>[27x]MSVHALRELFKHKGEKNYEVFSMEDFIGRLESEIGLNDSVVSQGRSLISSISHENFGTVQATDIQDAAAIYNKMQMLVNDYGFERVSSSDPQVRAREERVRENQITAATMAAIACADETKYIRALRGITKAKASNEDHVKVVQHQFNGPAGGIQVFENGVGLENYNEKSQRDFRVVTIGYNLAASRQDEFAERIYPTTVINPIEGGVVQVLPYIAVMKDVYHEVSGVKMDNEEVNMVEAYRDPSILDDESIALIPALDPAGSNADFFVDPALVPPYTIKNEQNLTITTAPLKANVRLDLMGNSNANLLIQRGMLEVSDTIDPAGRLKNLFVLLGGKVVKFKVDRLPRAVFQPDLVGDTRNAVIRFDSDDLVVSGDTTFIDGSADGVINDLKTAKLSLRLSVGFGGTISLSKGDSKFGATDTYVDKVLNEDGQVMDNADPAVKAILDQLTDLAVIGFELDTRFTNTNRRQRGHLLQTRALQFRHPIPMHAPVTLPMDTMTDEGPGEVVKALTVNTNIRNSNNAVKRMLNYLAQLREVVHNGYNRPKFGIIEGALSAVMRPTYRYKELDLEKVIDTIKSKDRWDDVCAAILNCVKAELFPAHRDSNIEAAFRVISGNQDETPMYLFCSDKEIANYLMTKGDDRTLGAYLKYDIVSTNNQLFDGKLVVIPTRAVQQENDILSWGQFFYVSTVIADLPITRGGHQVTREIAAIPFNLHVNNIPFALEFKITGFQKVMGETQFNGKLADLKP;> MAKRKARAVSAPVTLSEISEIPNEVTNAEDSVNELETTPTEIVSTESSENENTTADSENTAATDSTTDEESEDTSSTEANGDGESEEPDLSENQEDPKEPIETPEEPVEDDDGSGDPDGGTSEEKPTEGDPEDPEEPTEPTDPEEPTDPVDPVEPPPEEPKAFQLNLATVKSQFGDLPTYWAIELIKRYFSAPPAIYIPDVVDNPDFKIMVQQVKFFGNGLRPIYNSKNMITFTTMLEGASEATILEDMKKQQPALLSLLPWYDPNAEIDK;> MPTYIELINIVNDDTPEDDAVISDLMSQMNDKQTVLDSCRINHKGNAYFKFHVKGSISKDKLKALNETLKDSNLVVTDASTQRGFMPPNKFDDITYTEESVGYRAMVWTSFTIEKLLV;> MFLLPYETTVCKTLYNPTGGGKLYPKQYVDQIENAIKKANVYLPIPPVDARNGETLEHSGQITPVDDFEDIKKFTQIVNIGDRDNPKLVVDARLYKKIEQRTGIPRIIQQNEWQFQYIRMALNIKLLREGPDFLHRLGDIPVKVFYNWISGILTQKYSLPPESTQAIWVICAVYYFAMQDDDLTEPGQERDRLIPIISRLTYIPAGFIADVIDTLGPLHNAGDLAYEISTNGRSIRMGKLKFSDLQLLVSPSWFGTASRENVGVALEHMPTYITLIYMALADRSYRKTVLSQKVEMISRSDDASRFINLVNEAVSSQFVK;>MQQLGFELSRILKQLPNLGGSDRKTRAMLLANAVALQIPFETLLDFDEQQDKAVAKFKKILSKVNENIAVDTKLAVTYFNNILRIRQSLITGITDPCLVKAVLTSDTANDYLTVDDVNIVSAVVNGPDYNRIQADMGNALNQLIGSIDE[2x];> MSEVKPMSHVKEVDVEEEKLFFDENQPEMVEGEEETVSSASAPEVLAKMCVAVEAIHQLSDIYAITKLEGVSKPDVDGIRALVKRMSTEGFEAPKKAVASLEQYASMFTPTRSTLNVTISQEAVMATIINTLKTWFEKLMELFAKLIRWISDFKKRDVVVATRYGKIVRAVDQARTLFQELLVKNRLGNRKDA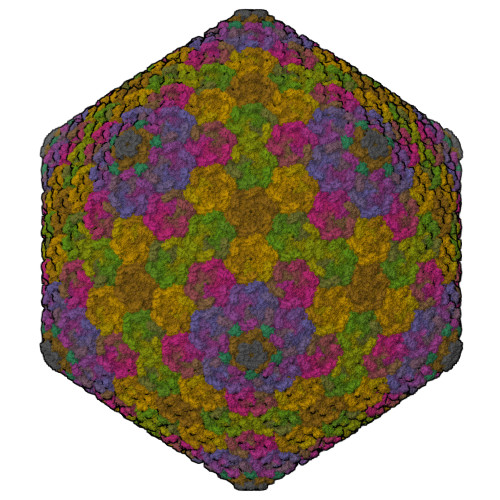LLEKFDAIAQSIIDDPKILASRIYAAAFGSVYYQKEIININNEARTELGTMEKLVGTIIEYVNYNGDDYRALMPIANIREIGKLATRCNELSTVYPDRSSIPDFPDKNFWKNSHLLKDRFVAPLDDLLKAYRNSSDALRKLKQLSRNYSQETIDAIGESVQLINTSLEGMRRITDTMFEYSQAQYLAASCVLNYYGKCAQVVSEDYKIHGFNDAIREWQRRFDKVIDDFKRGYAM;> MEGIDMPATNAVRPFGRNYSGGQQQAISRFTARPGDPQVEELYLIFTNFPAQTAYWEFHKKVLACAIRLFSGNYNWFILQDNNSNIDSYNYQFLLDTVRYIATGHRRISITQWPMLLATEPDAGAQLIEPRAEIATLFNELKLDLDTVSMIQNWVKHKNGMNDLMYTLHLLFGSVEVIDKD;> MSKPNLEWLASLESKEAKSTVDSSDMDNDQKEGSDKSQQDEATEPEKKITATDVQIAIEEYARIRALTTTKDLPTDPEPGDTYHVNGVDWIYQEDGGWVTMQGIYGHEHFDENGLNIEASGIDQKSGATKRYVVTGYNAQTNPAAMPGDNLTECVILMQNGLVPEVGVNGLTADCLLKIVKDLFEGYQAGPFACEENQVVINSMDRALSAIHQRLVRRKEQGTEGTYSGN;> MTQVLVMPKAVFESYKTAGVQFNKLLDTNYIVSETSVNDLAEIHQALTAFPFLLPEKLDIKLAVSPIIKVAELGEIDGPEQFKMKDLHNRLESRLATNELRDAGNRNLVYDYYLYPVDENLWVAVQQSAHIASSDPRRVSIQLNHTFFDSMINEMLNTRPRESVASTQIFTYYLESC;>MSLLKMLDKLSLESIEDQGTTIHGDVELVVENETSADVSSVLAEVDQIENNPVEEVLDADDAVQPTALDTEVTIVQAEDELGLIEDAKEALEKFQGLLLQAGEDGISRQAAAFMHVGMESIDRILGIEKSGLTAALENYDASPRSAIQKAAVISLEDLKEKLKEAGKKALEIIKKIVAMIKQKIKDFNPKLIALDMRITKTIDAIKSLKAGDLKKEEIKFTPSEYMVSSSGFIANNPKTIADFMTVFSTQYVSALRKYGELGVRYLKGDKSIDIDQVTSDLQAKMAEDINKAVEKAPGNVKLEVTSSKSGVNKWEVVEGDGETDLHEVEVDVRAPSKILAHLNILKGLVIKLQDFNKIDYKIAENLEKALADWNPDEAGMSKETARDALNIGGIDNSALVNYIAKCIAAQYTFIVKHELAAYGKETSKAPENDEK[3x];>MAKKKTVPAMDFFASLERVSDAEDKNVNLDVGKELPEQLKDDEDGKVNPCDEVTNVVTNTPIDVCKGPDVDGTADKINDKKIHVSQGLKEFQVAKGDRVENEITETADEMITKVSDTKDLNVSTKKPHQIADVPSNEDISIMEANETEQLDHGYDATALLETTEDIITGELDDHLESLSVEMFTIVNELTKVESVQTALENYIGLVSNRHHRGHDVDHDLAKAISIALESFDYKYFNNTVPSMESFISPLTRPKASIEVLDNLQAKAKEVSTVALDFIKKLIRIVVETYQRIRQNVSNQIERVNKIMKRVKENELPDEVRTIAIPRDLILGDTGESWVGVDPVQGVTVIRNLFDSIEKNGLRALKAALAGKTTDDKALALAKGMFGTATKINANGVRYASPVVPGNRVYTFGKDKAAVDFSILDAPGKPNYGITVELLVDKNVVMAQLKAVHNLLNHLNNIRGISKESTAEIIAQMTDKEATNVGKAYLTGTTEASNDLFKCVMIWITVLEKLVDSEIKETE[3x]>[3x]MFRVGILTVSDKGFRGERQDTTHLAIREVLAGGPFEVAAYELVPDEPPMIKKVLRLWADREGLDLILTNGGTG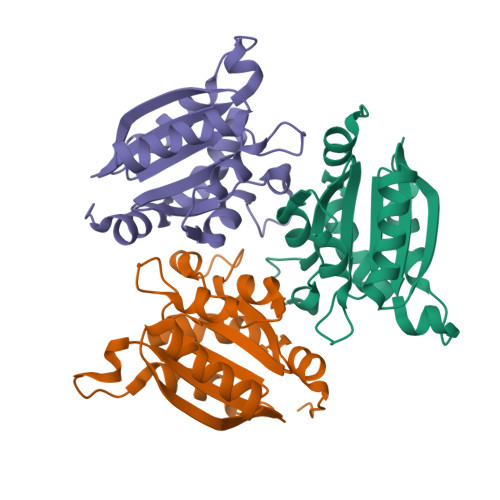LAPRDRTPEATRELLDREVPGLAELMRLVGLRKTPMAALSRGVAGVRGRTLILNLPGSPKGARESLEAVLPVLPHALSLVTGKPWKEGHHE> MPIFRFTALAMTLGLLSAPYNAMAATSNPAFDPKNLMQSEIYHFAQNNPLADFSSDKNSILTLSDKRSIMGNQSLLWKWKGGSSFTLHKKLIVPTDKEASKAWGRSSTPVFSFWLYNEKPIDGYLTIDFGEKLISTSEAQAGFKVKLDFTGWRAVGVSLNNDLENREMTLNATNTSSDGTQDSIGRSLGAKVDSIRFKAPSNVSQGEIYIDRIMFSVDDARYQWSDYQVKTRLSEPEIQFHNVKPQLPVTPENLAAIDLIRQRLINEFVGGEKETNLALEENISKLKSDFDALNIHTLANGGTQGRHLITDKQIIIYQPENLNSQDKQLFDNYVILGNYTTLMFNISRAYVLEKDPTQKAQLKQMYLLMTKHLLDQGFVKGSALVTTHHWGYSSRWWYISTLLMSDALKEANLQTQVYDSLLWYSREFKSSFDMKVSADSSDLDYFNTLSRQHLALLLLEPDDQKRINLVNTFSHYITGALTQVPPGGKDGLRPDGTAWRHEGNYPGYSFPAFKNASQLIYLLRDTPFSVGESGWNNLKKAMVSAWIYSNPEVGLPLAGRHPFNSPSLKSVAQGYYWLAMSAKSSPDKTLASIYLAISDKTQNESTAIFGETITPASLPQGFYAFNGGAFGIHRWQDKMVTLKAYNTNVWSSEIYNKDNRYGRYQSHGVAQIVSNGSQLSQGYQQEGWDWN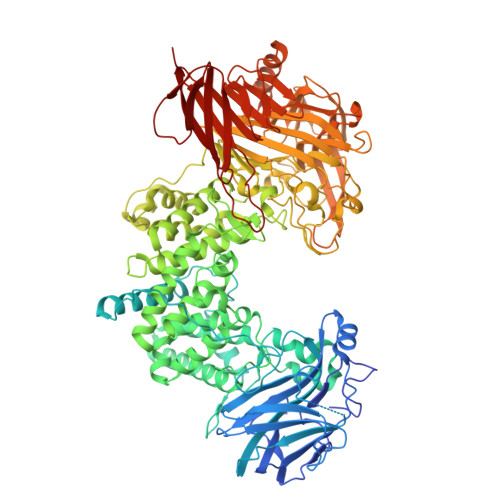RMEGATTIHLPLKDLDSPKPHTLMQRGERGFSGTSSLEGQYGMMAFNLIYPANLERFDPNFTAKKSVLAADNHLIFIGSNINSSDKNKNVETTLFQHAITPTLNTLWINGQKIENMPYQTTLQQGDWLIDSNGNGYLITQAEKVNVSRQHQVSAENKNRQPTEGNFSSAWIDHSTRPKDASYEYMVFLDATPEKMGEMAQKFRENNGLYQVLRKDKDVHIILDKLSNVTGYAFYQPASIEDKWIKKVNKPAIVMTHRQKDTLIVSAVTPDLNMTRQKAATPVTINVTINGKWQSADKNSEVKYQVSGDNTELTFTSYFGIPQEIKLSPLP>SAAATQAVPAPNQQPEVFCNQIFINNEWHDAVSRKTFPTVNPSTGEVICQVAEGDKEDVDKAVKAARAAFQLGSPWRRMDASHRGRLLNRLADLIERDRTYLAALETLDNGKPYVISYLVDLDMVLKCLRYYAGWADKYHGKTIPIDGDFFSYTRHEPVGVCGQIIPWNFPLLMQAWKLGPALATGNVVVMKVAEQTPLTALYVANLIKEAGFPPGVVNIVPGFGPTAGAAIASHEDVDKVAFTGSTEIGRVIQVAAGSSNLKRVTLELGGKSPNIIMSDADMDWAVEQAHFALFFNQGQCCCAGSRTFVQEDIYDEFVERSVARAKSRVVGNPFDSKTEQGPQVDETQFKKILGYINTGKQEGAKLLCGGGIAADRGYFIQPTVFGDVQDGMTIAKEEIFGPVMQILKFKTIEEVVGRANN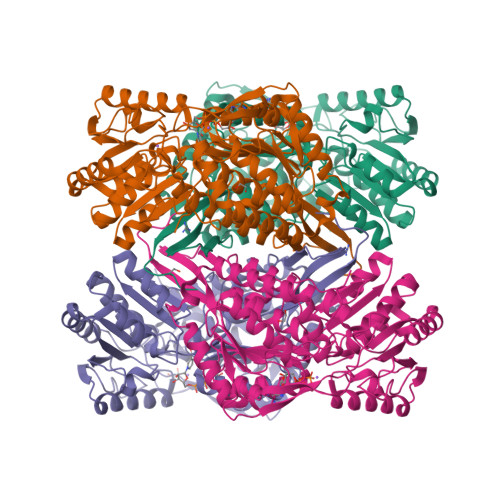STYGLAAAVFTKDLDKANYLSQALQAGTVWVNCYDVFGAQSPFGGYKMSGSGRELGEYGLQAYTKVKTVTVKVPQKNS[12x]>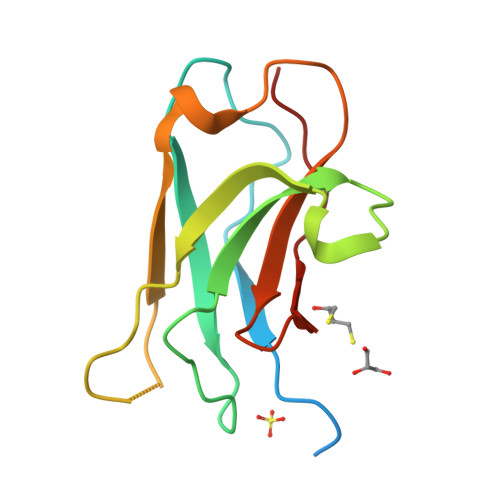[2x]MEETIKDPPTSAVLLDHCHFSQVIFNSVEKFYIPGGDVTCHYTFTQHFIPRRKDWIGIFRVGWKTTREYYTFMWVTLPIDLNNKSAKQQEVQFKAYYLPKDDEYYQFCYVDEDGVVRGASIPFQFR>GPRRVELDADATSGAFYARYRDGYVSGEPWPGAGPPPPGRVLYGGLGDSRPGLWGAPEAEEARRRFEASGAPAAVWAPELGDAAQQYALITRLLYTPDAEAMGWLQNPRVVPGDVALDQACFRISGAARNSSSFITGSVARAVPHLGYAMAAGRFGWGLAHAAAAVAMSRRYDRAQKGFLLTSLRRAYAPLLAR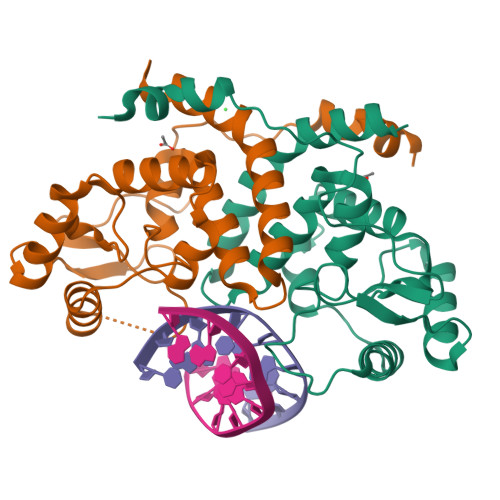ENAALTG[2x]>AGTLIGQVGVQM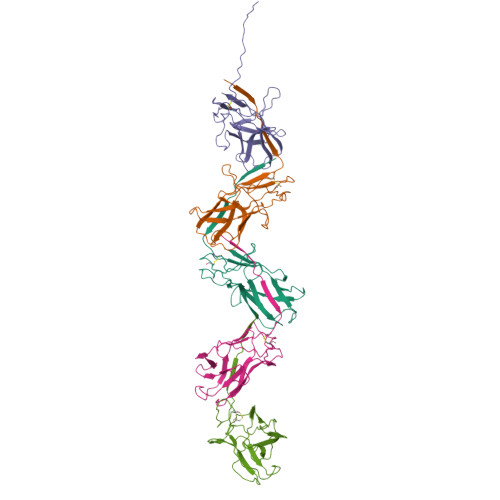VIGAGCTIINGSVSGGINQWGTLDFGSHSDLTNVVDAQTVGTSGNIQIQCSTGLTPSLTVNAGLHASGGQRYMQNTTTTSSTIAYNIYSDAARSALIQANTPVDISSVSTGTAVNIPLYGRVVPTGQSTPTPTAGTYTDTLLVTIAW[5x]>[2x]MAVTDLRDVEEDVKGKLDEWLNALVHLDKQQVERIYEELQGEMKHVLDFEIINYYKLLYTRYLIMKRDISALEEELDKLKKVYKKYSPFQKLLYMYGRGLLCCLQYRWKDGLDYLLKT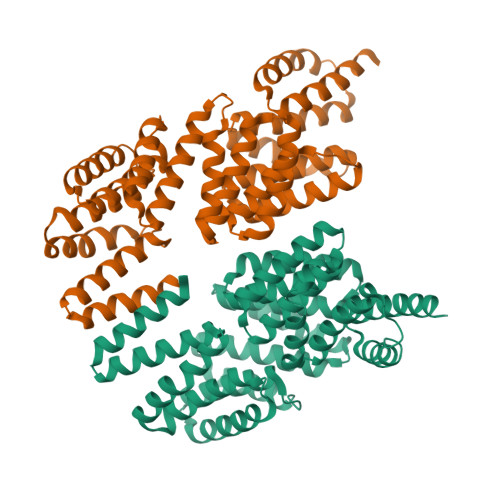EVMAKEQGYHETGLYYNIALAYTHLDIHHLAIHFVNMALEGFRSEAKARNIINCQILIAVSYTEKGQYEEALKMYESILREATSFADKDVLLAITLSNMGSIYYKKGKYQQAKKYYLDSLQLQKQIDLNYLDTIYEMALVCIKLEELEEARTLIDKGIDAAKQEERFNAKLYLLLMLRYKYFEEAKDYKAFLENEAIPLYKSAGNKIELKKVYVELAEHFSSLSRFEESNRYYRLVIDLMNDNKEERSHHHHHH> GSTIYHAKDAVQATKPDMRKPRLVVFVVGETARADHVSFNGYERDTFPQLAKIDGVTNFSNVTSCGTSTAYSVPCMFSYLGADEYDVDTAKYQENVLDTLDRLGVSILWRDNNSDSKGVMDKLPKAQFADYKSATNNAICNTNPYNECRDVGMLVGLDDFVAANNGKDMLIMLHQMGNHGPAYFKRYDEKFAKFTPVCEGN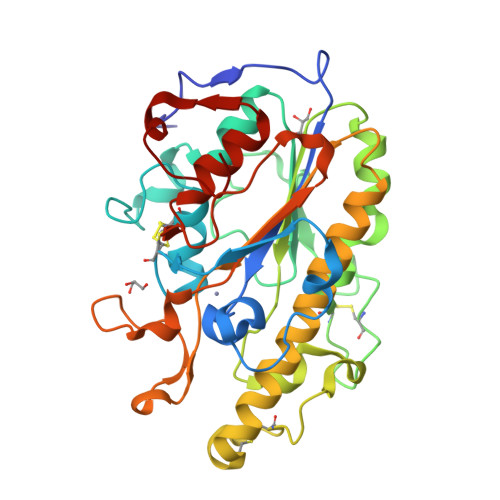ELAKCEHQSLINAYDNALLATDDFIAQSIQWLQTHSNAYDVSMLYVSDHGESLGENGVYLHGMPNAFAPKEQRSVPAFFWTDKQTGITPMATDTVLTHDAITPTLLKLFDVTADKVKDRTAFIR(2S)-2-cyclopentyl-2-phenyl-N-{[(2R,3R,4R,5R,6S)-3,4,5-trihydroxy-6-methylpiperidin-2-yl]methyl}ethanamide | C20 H30 N2 O4 | 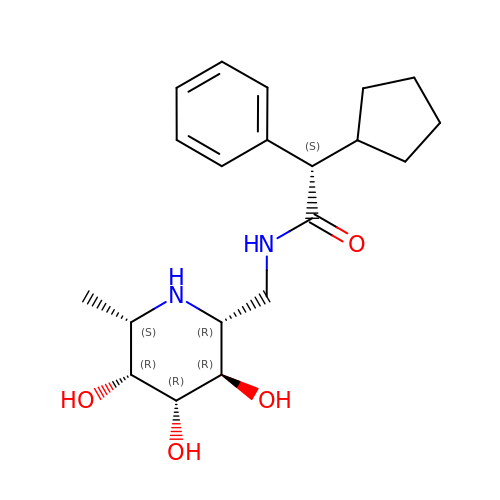USPGDBVOHJFDBD-YFRSTRBHSA-N pentyl 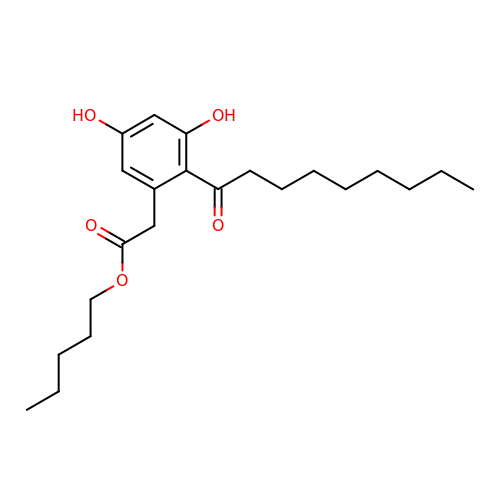(3,5-dihydroxy-2-nonanoylphenyl)acetate | C22 H34 O5 | FCKDHZVFIMRCNM-UHFFFAOYSA-N> MEDLYPSRQNNQPKILKRKDPVIYTDRSKDNQAPITKEQLDSYEKNGFLQIKNFFSEDEVIDMQKAIFELQDSIK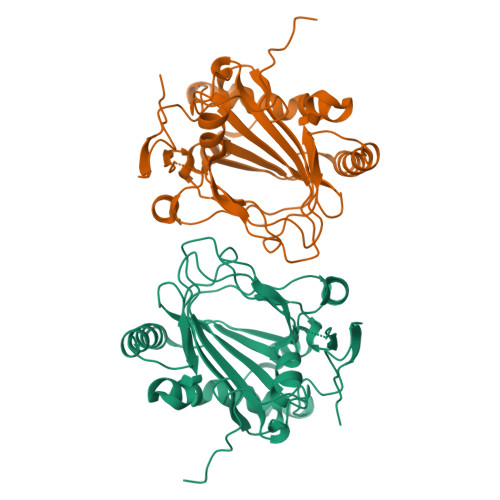DVASDKVIREPESNDIRSIFHVHQDDNYFQDVANDKRILDIVRHLLGSDVYVHQSRINYKPGFKGKEFDWHSDFETWHVEDGMPRMRAISVSIALSDNYSFNGPLMLIPGSHNYFVSCVGETPDNNYKESLKKQKLGVPDEESLRELTRIGGGISVPTGKAGSVTLFESNTMHGSTSNITPYPRNNLFMVYNSVKNRLVEPFSGGEKRPEYIAVREKQPVYSAVNSAWSHPQFEK> GIIMDSSISK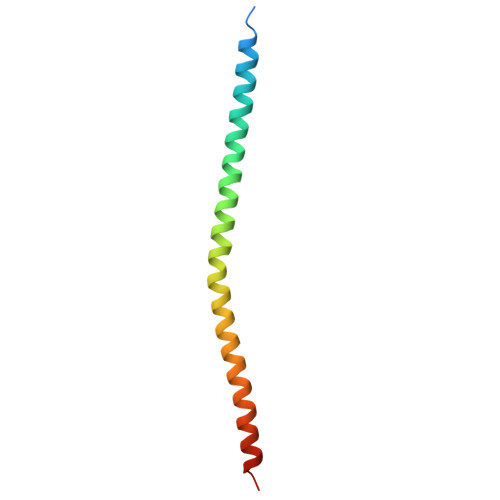QALSEIETRHSEIIKLENSIRELHDMFMDMAMLVESQGEMIDRIEYNVEHAVDYVERAVSDTKKAVKYQSKAR> MNPDLRKERASAT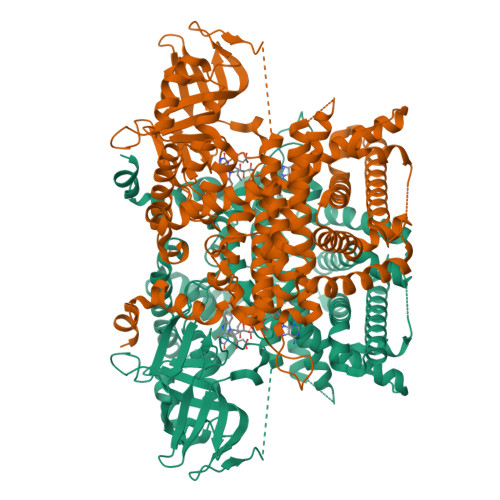FNPELITHILDGSPENTRRRREIENLILNDPDFQHEDYNFLTRSQRYEVAVKKSATMVKKMREYGISDPEEIMWFKNSVHRGHPEPLDLHLGMFLPTLLHQATAEQQERFFMPAWNLEITGTYAQTEMGHGTHLRGLETTATYDPKTQEFILNSPTVTSIKWWPGGLGKTSNHAIVLAQLITQGECYGLHAFVVPIREIGTHKPLPGITVGDIGPKFGYEEMDNGYLKMDNYRIPRENMLMKYAQVKPDGTYVKPLSNKLTYGTMVFVRSFLVGNAAQSLSKACTIAIRYSAVRRQSEIKQSEPEPQILDFQTQQYKLFPLLATAYAFHFVGRYMKETYLRINESIGQGDLSELPELHALTAGLKAFTTWTANAGIEECRMACGGHGYSHSSGIPNIYVTFTPACTFEGENTVMMLQTARFLMKIYDQVRSGKLVGGMVSYLNDLPSQRIQPQQVAVWPTMVDINSLEGLTEAYKLRAARLVEIAAKNLQTHVSHRKSKEVAWNLTSVDLVRASEAHCHYVVVKVFSDKLPKIQDKAVQAVLRNLCLLYSLYGISQKGGDFLEGSIITGAQLSQVNARILELLTLIRPNAVALVDAFDFKDMTLGSVLGRYDGNVYENLFEWAKKSPLNKTEVHESYHKHLKPLQSKL>[4x]GPGDPPATVYRYDSRPPEDVFQNGFTAWGNNDNVLEHLTGRSCQVGSSNSAFVSTSSSRRYTEVYLEHRMQEAVEAERAGRGTGHFI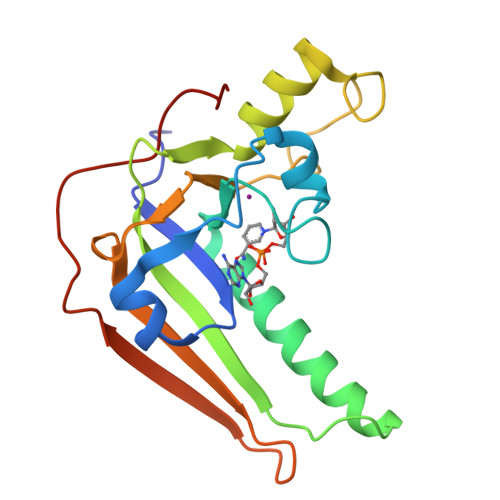GYIYEVRADNNFYGAASSYFEYVDTYGDNAGRILAGALATYQSEYLAHRRIPPENIRRVTRVYHNGITGETTTTEYSNARYVSQQTRANPNPYTSRR>MSLNERILLVDDDYSLLNTLKRNLSFDFEVTTCESGPEALACIKKSDPFSVIMVDMR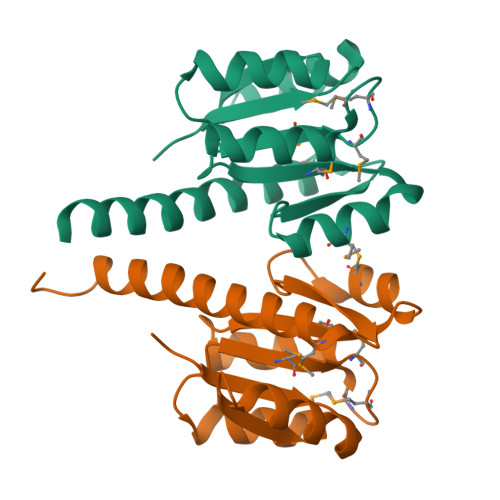MPGMEGTEVIQKARLISPNSVYLMLTGNQDLTTAMEAVNEGQVFRFLNKPCQMSDIKAAINAGIKQYDLVTSKEELLKKTFAGAISEGHHHHHH[2x]> PKFGTH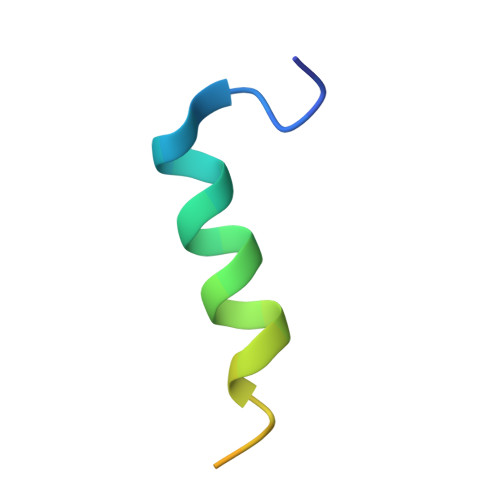HKALQEIRNSLLPFANETNSSRSTSE>MEFDDDLVDAEGNLVETGGTYYLLPHIWAHGGGIETAKTGNEPCPLTVVRSPNEVSKGEPIRISSQFLSLFIPRGSLVALGFANPPSCAASPWWTVVDSPQGPAVKLSQQKLPEKDILVFKFEKVSHSNIHVYKLLYC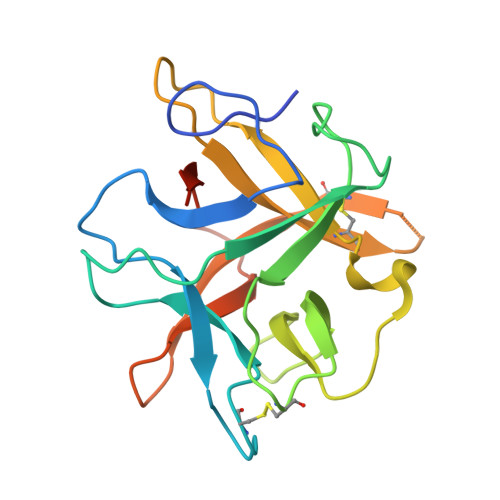QHDEEDVKCDQYIGIHRDRNGNRRLVVTEENPLELVLLKAKSETASSH[2x]>[8x]MALNEVALNCSFDNGKGLPWRVVNELTSGTAKGTVLFARPVSLFLNYKPQASQEAHELVIGGNWSGVGYPGPYGTVASDVKGIGYRISVDAQDGVKRVIPVDNQPHALDKRVTSFSGSTTSDYLQELVLTVDPGELPAGDLKVTSVSGSATLNLWAVDRLKGEASIGSVLAVPADNYPTGVCRKPYSLIGPASIAIGGGPPPPPIPKKCKVEVGREI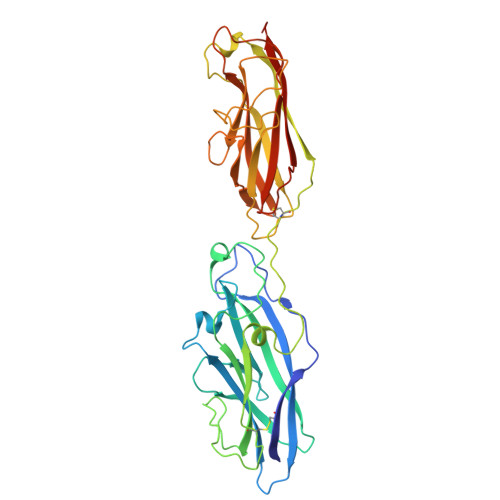NVKLGSVALKNFPRVNDTSTERSFDISLSECAALAKPEIAFRDKYVSAQQADPTILSLKSGGAAGFGIVVKNGLDQQRIRFDGTPYPMRRVGDSADLPLSAAYIRIGAEGELKAGVADGAAEFTFTFPSDNKVDGIVNFSGNITELEHHHHHH> MQDAITAVINSADVQGKYLDGAAMDKLKSYFASGELRVRAASVISANAATIVKEAVAKSLLYSDVTRPGGNMYTTRRYAACIRDLDYYLRYATYAMLAGDASILDERVLNGLKETYNSLGVPISSTVQAIQAIKEVTASLVGADAGK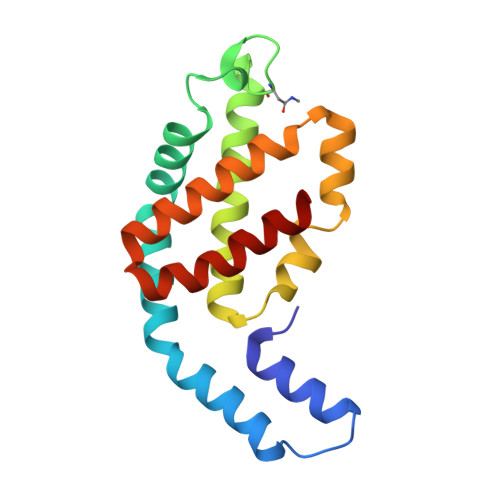EMGVYLDYICSGLS> EESYFSSSNRLDCVKANELCLKEPGCSSKYRTMRQCVAGRESNFSMATGMEAKDECRLVLDALKQSPLYNCRCKRGMKKEKNCLRIYWGIYQHLQGNDLLE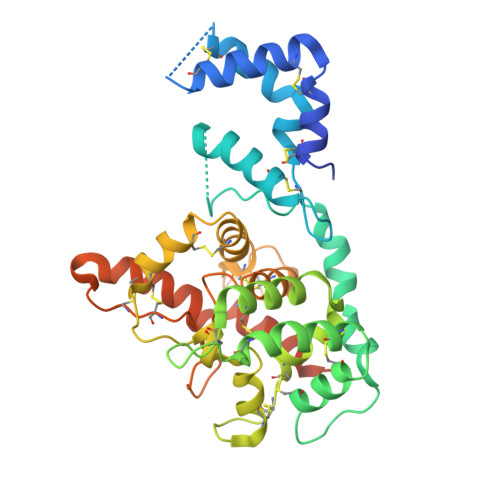DSPYEPVNSRLSDIFRLAPIYSGEPALAKENNCLNAAKACNLNDTCKKYRSAYISPCTSRVSTAEVCNKRKCHKALRQFFDKVPPKHSYGMLYCSCPLGDQSACSERRRQTIVPACSYEDKERPNCLTLQVSCKTNYICRSRLADFFTNCQPEPLSLSGCLKENYADCLLSYSGLIGTVMTPNYLRSPKISVSPFCDCSSSGNSKEECDRFTEFFTDNACLRNAIQAFGNGGSEFLEVLFQGPGGGENLYFQ>MGKVPHIRIENGAAIEEIYTFGRILGKGSFGIVIEATDKETETKWAIKKVNKEKAGSSAVKLLEREVNILKSVKHEHIIHLEQVFETPKKMYLVMELCEDGELKEILDRKGHFSENETRWIIQSLASAIAYLHNNDIVHRDLKLENIMVKSSLIDDNNEINLNIKVTDFGLAVKKQSRSEAMLQATCGTPIYMAPEVISAHDYSQQCDIWSIGVVMYMLLRGEPPFLASSEEKLFELIRKGELHFENAVWNSISDCAKSVLKQLMKVDPAHRITAKELLDNQWLTG[2x]

Men or mice with homozygous serine/threonine kinase 33 (STK33) mutations are sterile owing to defective sperm morphology and motility. STK33 is specifically required in male germ cells for spermatid differentiation, and Stk33 knockout male mice are sterile secondary to teratozoospermia and sperm immotility. STK33 is therefore considered a viable target with minimal safety concerns for contraception in men. To chemically evaluate STK33 for male contraception with STK33-specific inhibitors, we screened our multibillion-compound collection of DNA-encoded chemical libraries, uncovered potent STK33-specific inhibitors, determined the STK33 kinase domain structure bound with a truncated hit CDD-2211, and generated an optimized hit CDD-2807 that demonstrates nanomolar cellular potency (half-maximal inhibitory concentration = 9.2 nanomolar) and favorable metabolic stability.

There is a lack of available structures for STK33, which makes determining the molecular basis for our high-affinity STK33 inhibitors difficult. The STK33/CDD-2211 cocrystal contains one dimer per asymmetric unit, with each monomer showing clear density for bound CDD-2211. All residues in the construct are ordered except for a segment of the activation loop (residues 273 to 283 in chain A and 274 to 284 in chain B). As seen in other kinases with the exchanged activation segment conformation, the STK33 KD dimer is formed by the activation loop segment and the following two-turn helix with the APE motif from one monomer docking onto a surface formed between αE and αG helices of the other monomer. The biphenyl (BB3) binds to the outer lip of the active site near the hinge. It interacts with L122 and G123 on top and G198, E199, and M245 at the bottom through van der Waals interactions. The indazole (BB2) binds the ribose pocket and forms hydrogen bonds with backbones of E193 and C195 at the hinge region. The pyrrolidine with dimethyl amine (BB1) contacts the Mg2+ positioning loop, glycine-rich loop, and activation loop. The dimethyl amine forms a hydrogen bond with D265 that normally interacts with Mg2+. BB1 is shielded by F127 at the Gly-rich loop (top) and E242 and N243 at the catalytic loop (bottom), and it interacts with these residues through van der Waals interactions.>RMVDLPVIQPRLCTHARWPAPVYGLLVDPSLPSNPQWQNGRVHVDGTLLGTTPISGSWVSCFAAEAAYKFQSGTGEVATFTLIEQDGSAYVPGDRAAPLGYPDFSGQLEIEVQTETTKTGDKLKVTTFEMILGPTTNADQAPYQGRVFASVTAAASLDLVDGRVRAVPRSIYGFQDTIPEYNDGLLVPLAPPIGPFLPGEVLLRFRTYMRQIDTADAAAEAIDCALPQEFVSWFASNAFTVQSEALLLRYRNTLTGQLLFECKLYNEGYIALSYSGSGPLTFPTDGIFEVVSWVPRLYQLASV[4x];>[4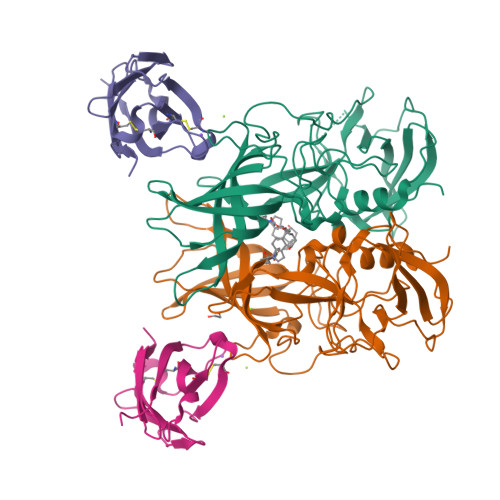x]EDPVTGPEEVSGQEQGSLTVQCRYTSGWKDYKKYWCQGVPQRSCKTLVETDASEQLVKKNRVSIRDNQRDFIFTVTMEDLRMSDAGIYWCGITKGGLDPMFKVTVNIGPVPT We therefore set out to characterize two previously unstudied proteins from the shipworm symbiont Teredinibacter turnerae that were initially identified by the presence of carbohydrate binding domains appended to uncharacterized domains with probable redox functions. One of these was TERTU_3803, which contained both a CBM10 and a CBM2 domain attached to a range of distinct modules (via flexible linkers) that did not bare any sequence similarity with catalytic domains typically found within carbohydrate-active enzymes. Using a ‘module walking’ approach, we searched for other genes coding for these X-domains. This led to the identification of TERTU_2913, which lacks CBMs but contains predicted X122, X183 and X132 domains. Taken together, these sequence analyses suggested that TERTU_3803 and TERTU_2913 could have a role to play in cellulose metabolism, and furthermore that role is likely to be a redox one given the presence of cytochrome domains within their linear amino acid sequences.

TtX183A, TtX183B and TtX183C, which all derive from TERTU_2913, were expressed and purified from the E. coli periplasm following co-expression with the cytochrome maturation machinery encoded on the pEC86 plasmid. All three proteins underwent crystal trials but only TtX183A and TtX183B formed diffracting crystals. The structure for TtX183A was determined via single-wavelength anomalous dispersion from the anomalous signal generated by the haem iron to a resolution of 1.4 Å. The resulting model was subsequently used to determine the structure of TtX183B via molecular replacement to 1.8 Å resolution. The polypeptide chain in each of TtX183A and TtX183B fold around the haem to produce a tertiary structure dominated by α-helices, as expected for small c-type cytochromes [Fig. 2(a)]. To examine the structural similarities within our TtX183 domain structures, we compared TtX183A with TtX183B and found that the structures superposed with one another with an r.m.s.d. of 1.12 Å over 59 Cα positions. In the structures of TtX183A and TtX183B, the haem propionate groups are highly solvent exposed where in CjX183 a loop was found to interact with these groups. This is likely to provide an easier exit route for electrons when O2 is present, explaining the apparent lack of stability of the reduced state for the TtX183s compared with CjX183.

>[3x]GYVGNAANGQLLYANATLDCTNCHGAMGDGLYKIDPHATVFGQNNKTLENIIAEDMPQLNPASCGAECAADIAAYIRTWAGLEHHHHHH(~{E})-~{N}-[4-[2-(4-oxidanylpiperidin-1-yl)pyridin-4-yl]pyridin-2-yl]-3-phenyl-prop-2-enamide | C24 H24 N4 O2 | 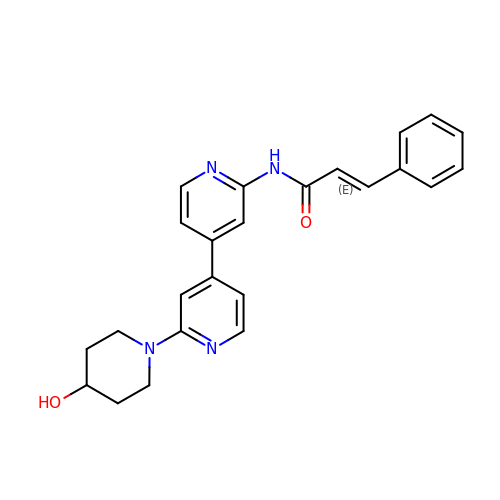LLCXZJGKTNDVLE-UHFFFAOYSA-N>MKGTFVGTWIKTLRDLYGN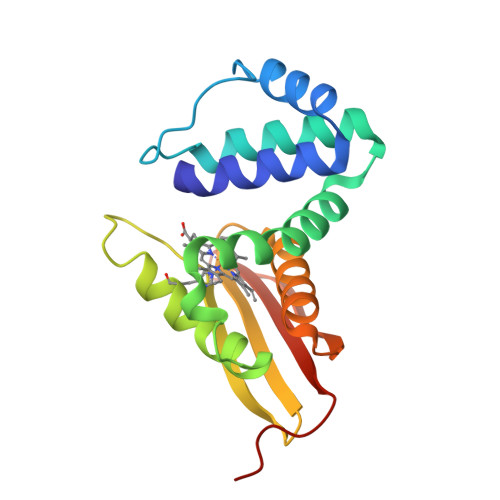DVVDESLKSVGWEPDRVITPLEDIDDDEVRRIFAKVSEKTGKNVNEIWREVGRQNIKTFSEWFPSYFAGRRLVNFLMMMDEVHLQLTKMIKGATPPRLIAKPVAKDAIEMEYVSKRKMYDYFLGLIEGSSKFFKEEISVEEVERGEKDGFSRLKVRIKFKNPVFEYKKN[2x]> GSAMGTGERGLFVAAGNSRRKITYFGTLTQKAPNWYRCSSTRAKEEVVGHVTLNKEHPDMTIECVDDGLGGEFLPLEGARSSYPRVCHIDAKDQDDC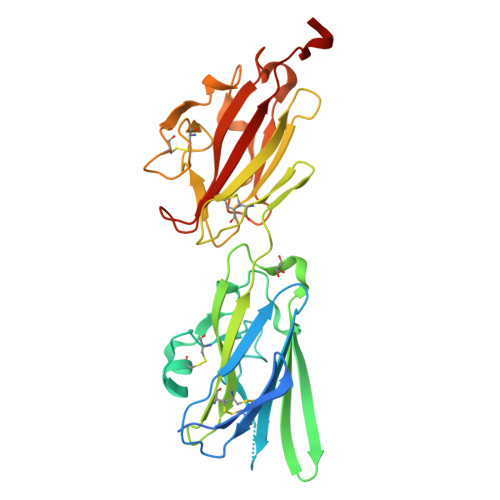ERNRGFLTDYIPGAKQYWYKIEKVEQNGEQSVLYKFTVPWILLPPAKQRYKVGCRYPNHEYCFVEVTVEPTPPMVEGKRVTCGYSESGPVNLEVDLSKNANFIEIRCGEQHHPQPSTYTLQYCSGDSVDPQKCSPQSLTNIFYDYSSSWWKGKLNGPDGATLTIPPGGFPEEDKSFLVGCSLTVDGPPFCNVKVRVAGNPAAALVPR>GKSDKIIPIAENKEAKAKYDILETYEAGIVLKGSE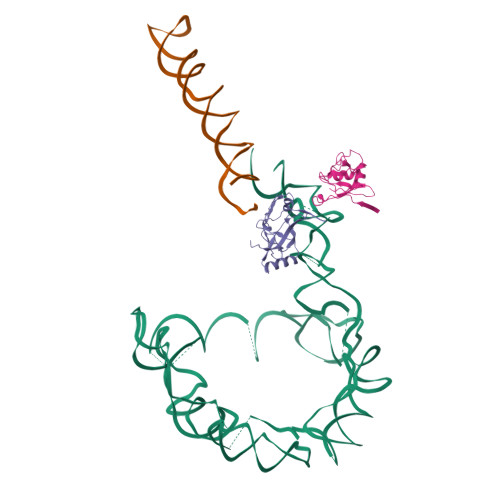VKSLREKGTVSFKDSFVRIENGEAWLYNLYIAPYKHATIENHDPLRKRKLLLHKREIMRLYGKVQEKGYTIIPLKLYWKNNKVKVLIALAKGKKLYDRRRELKEKAMKRELEREFKGKIHL[2x]> QKEGVLRVITRNSPATYFQDRNGETGFEYELAKRFAERLGVELKIETADNLDDLYAQLSREGGPALAAAGLTPGREDDASVRYSHTYLDVTPQIIYRNGQQR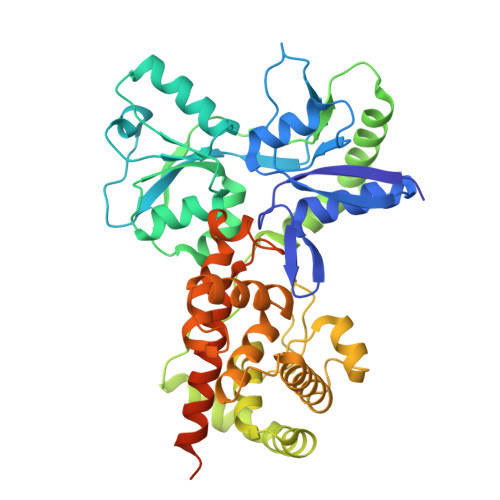PTRPEDLVGKRIMVLKGSSHAEQLAELKKQYPELKYEESDAVEVVDLLRMVDVGDIDLTLVDSNELAMNQVYFPNVRVAFDFGEARGLAWALPGGDDDSLMNEVNAFLDQAKKEGLLQRLKDRYYGHVDVLGYVGAYTFTQHLQQRLPRYESHFKQSGKQKDTDWRLLAAIGYQESLWQPGATSKTGVRGLMMLTNRTAQAMGVSNRLDPKQSIQGGSKYFVQIRSELPESIKEPDRSWFALAAYNIGGAHLEDARKMAEKEGLNPNKWLDVKKMLPRLAQKQWYAKTRYGYARGGETVHFVQNVRRYYDILTWVTQPQMEGSQIAESGLHLPGVNKTRPEEDSGDEKL> GSHMASPNGQTKPLPALKLALEYIVPAMNKHGICVVDDFLGKETGQQIGDEVRALHDTGKFTDGQLVSQKSDSSKDIRGDKITWIEGKEPGCETIGLLMSSMDDLIRHCNGKLGSYKINGRTKAMVACYPGNGTGYVRHVD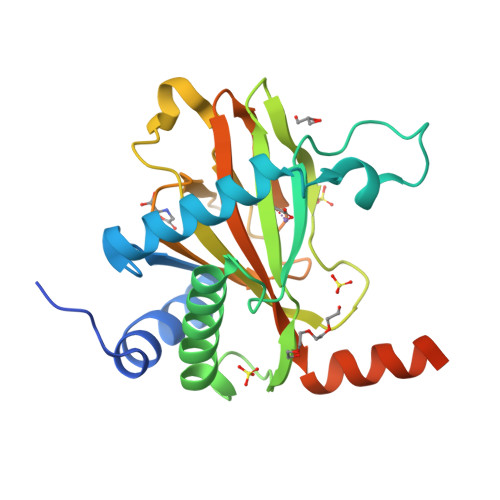NPNGDGRCVTCIYYLNKDWDAKVSGGILRIFPEGKAQFADIEPKFDRLLFFWSDRRNPHEVQPAYATRYAITVWYFDADERAAAKVKYLTGEKGVRVELNKPSDSVGKDVF> MDKINLVCGSLLHNIGKIIYRGTSERAKHSKLGGDFIKSFEQFRNTELTDCIRYHHAQEITSVKSNKEKNSLFYITYIADNISSGMDRRKDLEEGAEGFNWDKKVALGSVFNVLNEKEKGRQNYSYPFVARTRIKEEPLNFPTATQNQYTTSYYDGLITDMKTILQRLKPDKEHINSLLQMMESLWSYVPSSTDKNQLVDISLYDHSRTTAAIASAIYDYFQAENITDYQKELFDYNATEFYDKNAFLMMNFDMSGVQNFIYNISGSKALKSLRARSFYLDMLLEYISDNLLEKLELSRANILYVGGGHAYLLLANTNKTKAILSDFEHDLKTWFLDKFKIDLYVAMAYTEVSANDLMNHNGHYRDIYRRLSQKTSAKKANRYTAEEILNLNHQGTENARECRECKRSDLLIEEDDICEICDSLQKVSRDLTRENIFVIANEGVLDMPFGKKMSALSYSQADKLKKSNAEVQIYAKNISEIGQNLMTRIDMGDYTYRSDFHEMLEEVEVGINRLGVLRADVDNLGQAFINGIPDDYLSISRTATFSRAMSRFFKNYLNQLLAEKSYKINVIYAGGDDLFMIGAWQDILDFSIVLKQKFADFTQNKLSISAGIGMFREKYPVARMASLTGDLEDAAKDYKPDERAVQATKNAVTLFDATNVFSWDTLENDIFVKLDAITKNFEKLDETGKAFIYRLIDLLRGVNENQQINIARLAYTLSRMEEKIGKTFAQELYNWANADRKTLIMALEIYILKTR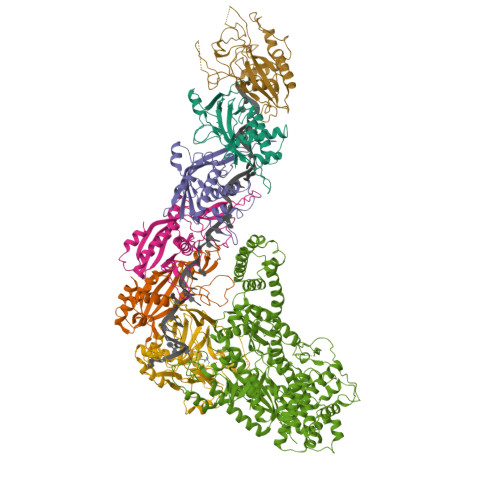E;> MKIIKLYFESPVHFGEKRLSESKITFSADTLFSALMIEAVGLGKEDEFYQLASNNLVKFSDAFPFIDQYYYIPKPMFNLKLEKEDENPSKAFKKLLYVPIDSLEDYLSGGLDAYFERESFNLGKLALSEKVQQHDFKDSEPYNVGTFTFKENTGLYVLIEQTHPLLEELLENLQYSGIGGKRNSGYGKFKFEILEDSDIEDLFSAKGNRKILLSGALPKDAELEQALKNASYLLERRGGFVQSDTYATNLVKKQDLYVFKSGSTFENSFDGDIYQVGKKGNHPVYKYAKSFFLEVS;>[4x]MKLVIEGTIVLKTGMHIGGSSDFSAIGAVASPVVRDTLTRLPLIPGSSLKGKMRYLLAKELNNGILLNEPNNDQDEILRLFGSSEKDKIRRARLKFNDIKLSNLAELETFNVSSTEVKFENTINRKTAVANPRQIERVIAGSKFDFEIFYNLDDIKEVEKDFENIKQGFDLLEFDYLGGHGTRGSGRIAFENLSVITAVGNFEKINTLNEILGA;> MKKTYRVTLTALGPIFIGGGEKLKKYEYIFDKQKKVAHMIDHTKFTKYLLEKNLLDDFTSRVNSHFDLYDYLVNKKGIVFMPLVKYSVPVAQFRTEVKNRFGKPISSPPMNDLNTFVKDAFGRPYIPGSSLKGALRTAILNDLKEDTKENEVFAHLQVSDSETIDLENLKVYQKVDYSKTAKPLPLYRECLKPNTEITFTVSFDDEYLTLKKIQNALHKTYQHYYIKWLKGGKVGETLIKGVYDSHADELKKNTFALDQPSQNQGEIIYIGGGAGFVSKTLHYKSKNRDQARNDSFDILKQLFRTTYSKMRSVPDNVPVALKLAVETKTFNGRVTGKHYLEMGKARIKLEEL Collagen prolyl 4‐hydroxylase (C‐P4H) catalyzes the 4‐hydroxylation of Y‐prolines of the XYG‐repeat of procollagen. The α‐subunit provides the N‐terminal dimerization domain, the middle peptide‐substrate–binding (PSB) domain, and the C‐terminal catalytic (CAT) domain. There are three isoforms of the α‐subunit, complexed with a β‐subunit that is protein disulfide isomerase, forming C‐P4H I‐III. The PSB domain of the α‐subunit binds proline‐rich peptides, but its function with respect to the prolyl hydroxylation mechanism is unknown.

In addition, it is shown here by crystallographic binding studies that the POG‐PAG‐POG peptide (with 4‐hydroxyprolines at Y‐positions 2 and 8) also adopts the PxGP mode of binding to PSB‐I as well as to PSB‐II. Calorimetric binding studies show that the affinities of these peptides are lower for PSB‐I than for PSB‐II, with, respectively, K D values of about 70 μM for PSB‐I and 20 μM for PSB‐II.

> MHHHHHHMLSVDDCFGMGRSAYNEGDYYHTVLWMEQVLKQLDAGEEATTTKSQVLDYLSYAVFQLGDLHRALELTRRLLSLDPSHERAGGNLRYFEQLLEEE;> PPGPAGPPG> KKATQ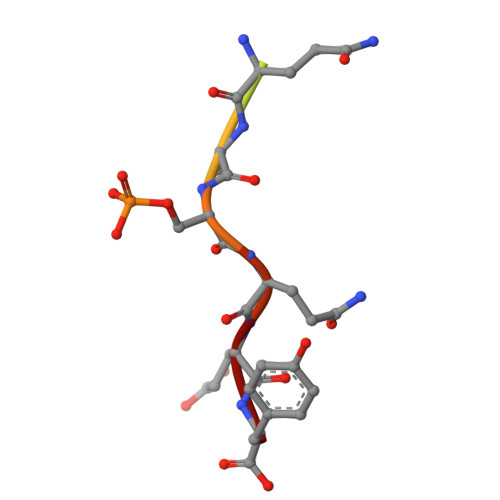ASQEY>[2x]GPGSMKIDVVTIFPEYLQPVRQSLPGKAIDAGLVDVAVHDLRRWTHDVHKSVDDSPYGGGPGMVMKPTVWGDALDEICTSETLLVVPTPA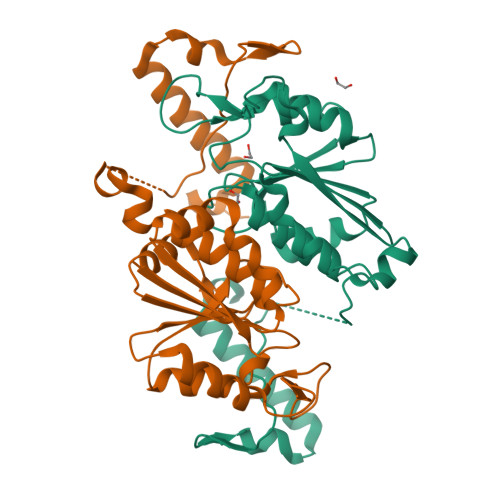GYPFTQETAWQWSTEDHLVIACGRYEGIDQRVADDAATRMRVREVSIGDYVLNGGEAAALVIIEAVLRLVPGVLGNALSAQEDSHSEGMASLLEGPSYTRPPSWRGMDVPPVLLSGDHAKIAAWRAEQSRQRTIERRPDLLGFDSPTGEHGGDGLS> ANS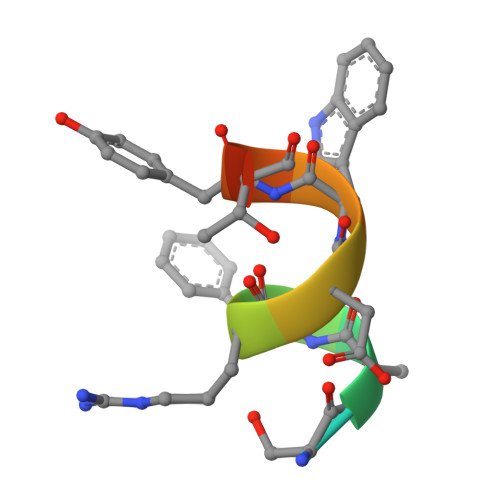SFRDWYTSS>[2x]MSTGEAIPRVAVVVFILNGN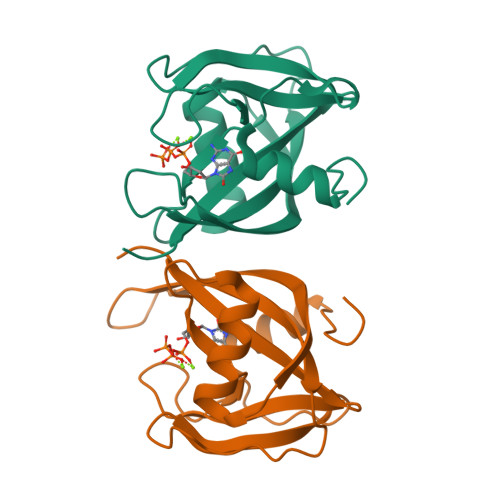SILLGRRRSSIGNSTFALPGGHLEFGESFEECAAREVMEETGLKIEKMKLLTVTNNVFKEAPTPSHYVSVSIRAVLVDPSQEPKNMEPEKCEGWDWYDWENLPKPLFWPLEKLFGSGFNPFTHGGGD>SMPEAPKIAALEVSDESLAEKNKNKLQFIEDVTTNADDVQRRVLEEILSRNADVEYLKRHGLEGRTDRETFKHIMPVVTYEDIQPEINRIANGDKSQVLCSNPISEFLTSSGTSGGERKLMPTIEEELDRRSLLYSLLMPVMDQFVPGLDKGKGMYFLFIKSESKTPGGLPARPVLTSYYKSSHFKNRPYDPYTNYTSPNQTILCSDSYQSMYSQMLCGLCQHKEVLRVGAVFASGFIRAIKFLEKHWPELARDIRTGTLSSEITDSSVREAVGEILKPDPKLADFVESECRKTSWQGIITRLWPNTKYVDVIVTGTMSQYIPTLDYYSNGLPLVCTMYASSECYFGVNLRPLCKPSEVSYTLIPNMAYFEFLPVHRNSGVTSSISLPKALTEKEQQELVDLVDVKLGQEYELVVTTYAGLYRYRVGDVLSVAGFKNNAPQFSFICRKNVVLSIDSDKTDEVELQNAVKNAVTHLVPFDASLSEYTSYADTSSIPGHYVLFWELCLNGNTPIPPSVFEDCCLTIEESLNSVYRQGRVSDKSIGPLEIKMVESGTFDKLMDYAISLGASINQYKTPRCVKFAPIIELLNSRVV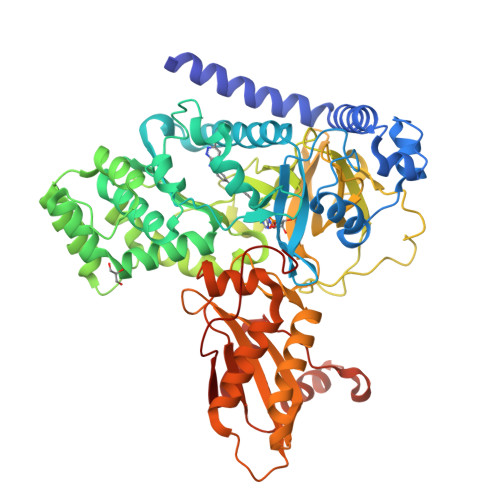DSYFSPKCPKWSPGHKQWGSN[2x]> SSQIRQNYSTEVEAAVNRLVNLYLRASYTYLSLGFYFDRDDVALEGVCHFFRELAEEKFEGAERLLKMQNQRGGRALFQDLQKPSQDEWGTTLDAMKAAIVLEKSLNQALLDLHALGSAQADPHLCDFLESHFLDEEVKLIKKMGDHLTNIQRLVGSQAGLGEYLFERLTLKHD

As a scaffold for aromatic cluster design, we chose ferritin as a protein cage platform with a 12 nm outer diameter and an 8 nm inner cavity, composed of 24 subunits. To prove this concept through protein engineering, we focused on a two‐fold symmetric inter‐subunit interface of a recombinant horse spleen apo‐L ferritin (Fr) as a target region for mutagenesis. Herein, we present the construction of an aromatic cluster with an artificial molecular binding pocket at the two‐fold symmetric interface of ferritin and explore its ligand‐binding characteristics. We developed a system that uses ligand binding as a driving force to induce and propagate changes in the orientation of multiple aromatic side chains.

To create the ligand‐binding pocket, we first designed a mutant Fr‐F1 (Fr‐R59F) in which Arg59 was replaced by Phe59. Analysis of the 2Fo‐Fc maps revealed electron densities corresponding to Nile Red (NR) at the two‐fold symmetric interfaces of NR•Fr‐F1, NR•Fr‐F2, NR•Fr‐F4, and NR•Fr‐F6, observed as overlapping densities due to the interface symmetry. NR was positioned between two F59 residues, forming π–π stacking interactions in an F59–NR–F59' configuration. Anion‐π interactions between NR and E60 in NR•Fr‐F1 and NR•Fr‐F2, and CH‐π interactions between NR and F60 in NR•Fr‐F6, were identified, indicating NR's stabilization in the F59–F59' pocket via multiple non‐covalent interactions. Notably, NR•Fr‐F1 and NR•Fr‐F2, containing only one and two Phe residues, respectively, achieve higher quantum yields (94 and 95%, respectively) and longer lifetimes (5.54 and 5.75 ns, respectively) than NR•Fr‐F6 with six Phe residues per monomer. The hydrophobic and polar nature of the protein surface around NR influences its fluorescence properties, with the partially polar microenvironment in Fr‐F1 and Fr‐F2, attributed to Glu residues near the pocket entrance, potentially enhancing fluorescence. The quantum yield of Nile Red (NR) significantly increased from 0.50 in 100% methanol (MeOH) and 0.38 in a 50% MeOH‐water mixture to 0.88–0.95 upon encapsulation within Fr‐F1, Fr‐F2, Fr‐F4, and Fr‐F6. Furthermore, NR's fluorescence lifetime extended from 2.87 ns in organic solvent and 1.26 ns in aqueous‐organic mixture to 5.23–5.75 ns within these ferritin variants.>GHMPLQPIPGVASVSPANGAVVGVAHPVVVTFTTPVTDRRAVERSIRISTPHNTTGHFEWVASNVVRWVPHRYWPPHTRVSVGVQELTEGFETGDALIGVASISAHTFTVSRNGEVLRTMPASLGKPSRPTPIGSFHAMSKERTVVMDSRTIGIPLNSS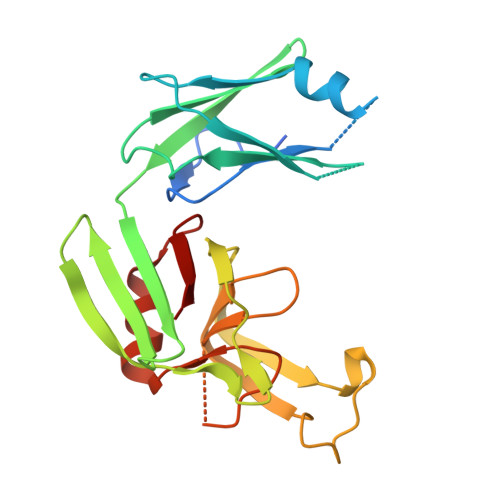DGYLLTAHYAVRVTWSGVYVHSAPWSVNSQGYANVSHGCINLSPDNAAWYFDAVTVGDPIEVVG[4x]>MSLRVYVTGNITVDETWSIPDIPKKGASIHGVKVSQDIGGKGANQAIILSRCGIETRLIAATGNDSNGAWIRQQIKNEPLMLLPDGHFNQHSDTSIILNSADGDNAIITTTAAADTFSLDEMIPHMADAVAGDILLQQGNFSLDKTRALFQYARSRGMTTVFNPSPVNPDFCHLWPLIDIAVVNESEAELLQPYGVKTLVITQGAAGAWLVQEGQRQFCPAVPAEALDTTGAGDTFLAVMLASALLRGVAPDALALAHASRAAAITVSRRGTLSAFPGSRELAALLTTDGA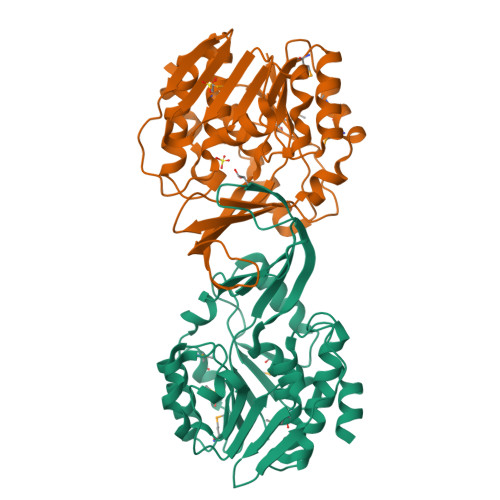EGHHHHHH[4x]>[4x]GPHMRKQEIIKTTEQLIEAVNNGDFEAYAKICDPGLTSFEPEALGNLVEGMDFHRFYFENL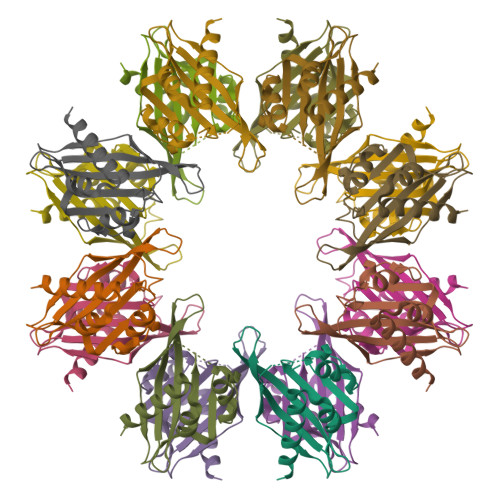LAKNSKPIHTTILNPHVHVIGEDAACIAYIRLTQYIDGQGRPRTSQSEETRVWHRRDGKWQNVHFHCSGAPVAPLQ>[2x]AEAGITGTWYAQLGDTFIVTAGADGALTGTYEAAVGNAESRYVLTGRYDSAPATDGSGTALGWTVAWKNNYRNAHSATTWSGQYVGGAEARINTQWLLTSGTTEANAWKSTLVGHDTFTKVKPSAAS;>AEAGITGTWYNQLGSTFIVTAGADGALTGTYESAVGNAESRYVLTGRYDSAPATDGSGTALGWTVAWKNNYRNAHSATTWSGQYVGGAEARINTQWLLTSGTTEANA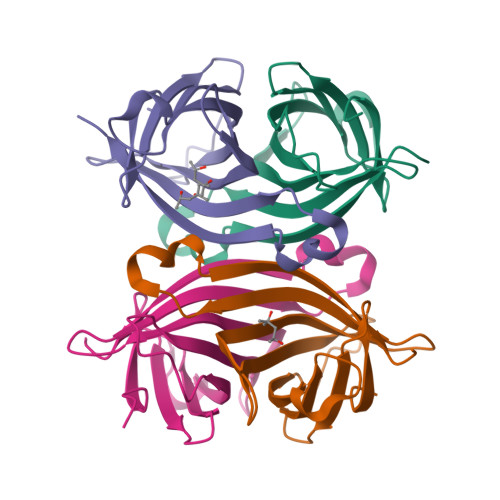WKSTLVGHDTFTKVKPSAASEEEEEE[2x]>MAHHHHHHMMSKPHHATLESIKYTPGSLRLLDQRKLPLETVFDDVLTVEDIWSAIKEMRVRGAPAIAVSAALGIAVATQRKAANGELKSGREVQTFLLTSCDFVMTSRPTAVNLFNCLRDLKAQVDKLDPTKAAAEVAQAFVELAEAVYTNDVAFNEGIMRHGAAHILAAAKAEGRDKVSILTICNTGALATSRYGTALGVVRQLFYDGKLERVYACETRPWNQGARLTVYECVQEDIPCTLICDGAASSLMLNRKIDAVVVGADRICQNGDTANKIGTYNLAVSAKFHGVKLYVAAPTTTLDVKTASGNHVEIEEREPTEITTNLVTKQRVVADGPHLSIW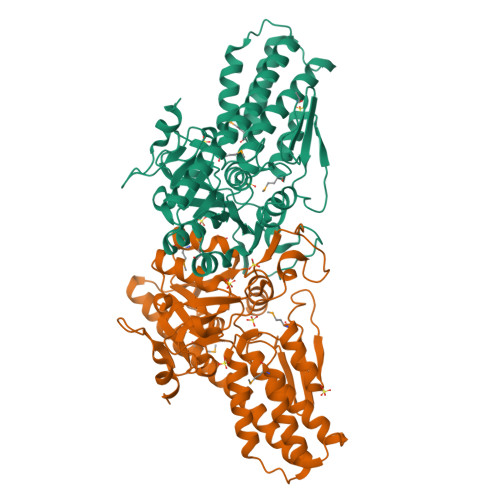NPVFDITPSELITGGIITEKGVQAPAASAPYYDIASIIAQA[2x]>[2x]MHHHHHHFNLPPGNYKKGGQYLRINPDGTVDGTRDRSDTHIQFQISPEGNGEVLLKSTETGQYLRINPDGTVDGTRDRSDTH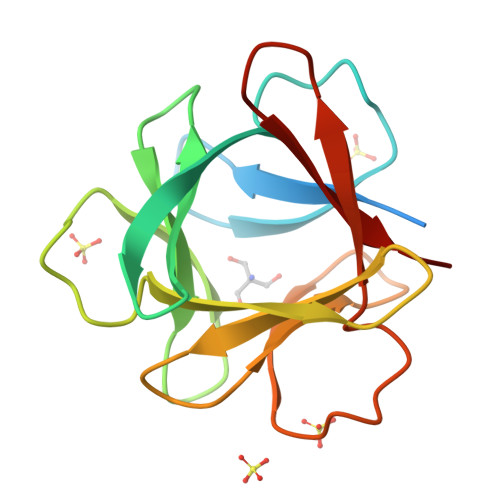IQFQISPEGNGEVLLKSTETGQYLRINPDGTVDGTRDRSDTHIQFQISPEGNGEVLLKSTE>MSLERPEEYLPNIFEGKKGVIVDYGCGNGFYCKYLLEFATKLYCIDINVIALKEVKEKFDSVITLSDPKEIPDNSVDFILFANSFHDMDDKQHVISEVKRILKDDGRVIIIDWRKENTGIGPPLSIRMDEKDYMGWFSNFVVEKRFNPTPYHFGLVL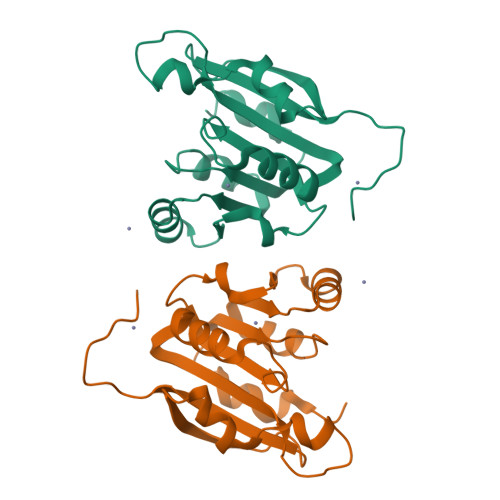KRKTSEGHHHHHH[2x]>MTGSSPALNARQQALLTALNACGDEMSGQQLHRSLDDEASMGLATVYRNLRQLQQRGLVRCRHLPTGEALYAPVDRDRHHLTCVDCGTTQVLDHCPIHGIDVPADSRGDFELLFHTLEFFGFCSSCRPQRSSKP[4x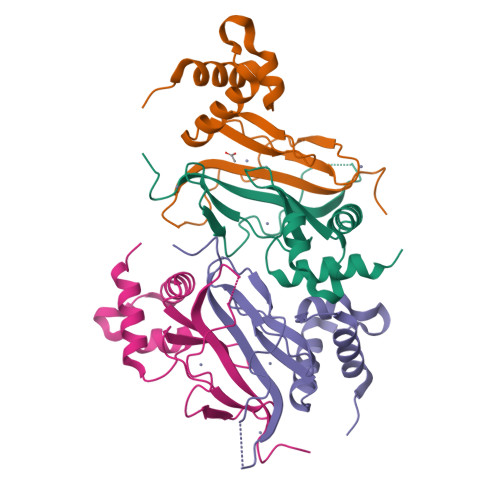]> GPDSMRVTQEEIKKEPEKPIDREKTCPL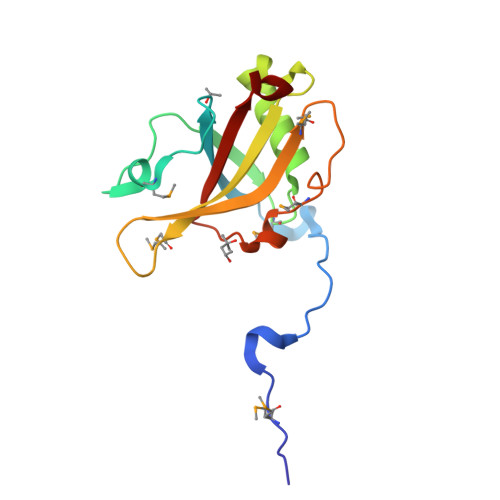LLRVFTTNNGRHHRMDEFSRGNVPSSELQIYTWMDATLKELTSLVKEVYPEARKKGTHFNFAIVFMDLKRPGYRVKEIGSTMSGRKGTDDSMTLQSQKFQIGDYLDIAITPPNRA> GSHMSQSNRELVVDFLSYKLSQKGYSWSQFSDVEENRTEAPEETESAVKQALREAGDEFELRYRRAFSDLTSQLHIT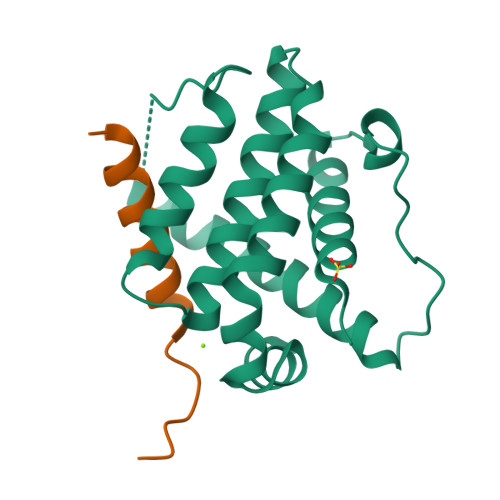PGTAYQSFEQVVNELFRDGVNWGRIVAFFSFGGALCVESVDKEMQVLVSRIASWMATYLNDHLEPWIQENGGWDTFVDLYG;> EEIIHKLAMQLRHIGDNIDHRMVRED BENZIMIDAZOLE | C7 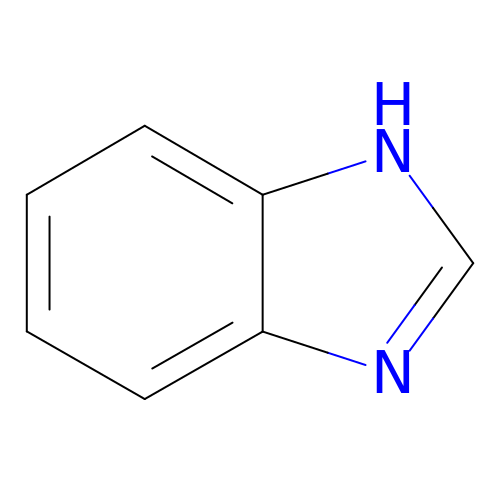H6 N2 | HYZJCKYKOHLVJF-UHFFFAOYSA-N> RILPEVKVEGELGGSVTIKCPLPEMHVRIYLCREMAGSGTCGTVVSTTNFIKAEYKGRVTLKQYPRKNLFLVEVTQLTESDSGVYACGAGMNTDRGKTQKV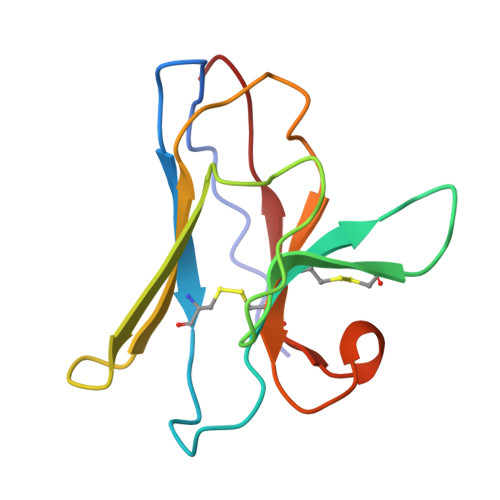TLNVHS> GSIPHKENMFKSKHKLDFSLVSMDQRGKHILGYADAELVNMGGYDLVHYDDLAYVASAHQELLKTGASGMIA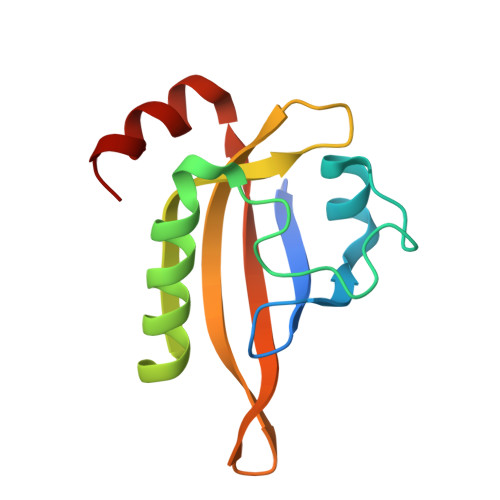YRYQKKDGEWQWLQTSSRLVYKNSKPDFVICTHRQLMDEEGHDLLGKR> GITALRQQVETLQGQVQRLQKAFSQYKKVELFP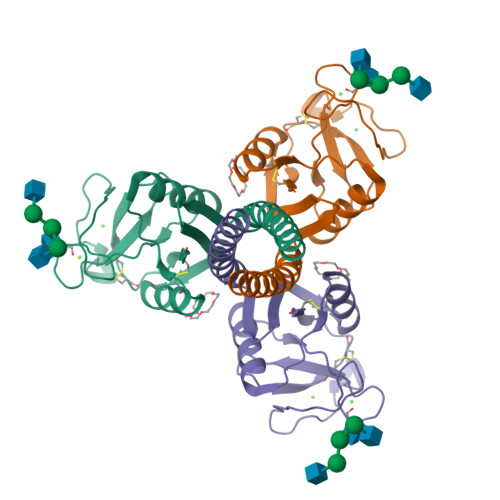NGRGVGEKIFKTGGFEKTFQDAQQVCTQAGGQMASPRSETENEALSQLVTAQNKAAFLSMTDIKTEGNFTYPTGEPLVYANWAPGEPNNNGGSSGAENCVEIFPNGKWNDKACGELRLVICEF> GSHMGTAAEHHREGIMSQFFYIHPDNPQQRLINQAVEIVRKGGVIVYPTDSGYALGCKIEDKNAMERICRIRQLPDGHNFTLMC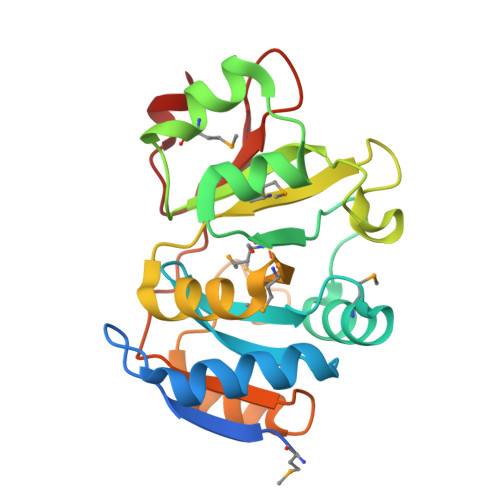RDLSELSTYSFVDNVAFRLMKNNTPGNYTFILKGTKEVPRRLLQEKRKTIGMRVPSNPIAQALLEALGEPMLSTSLMLPGSEFTESDPEEIKDRLEKQVDLIIHGGYLGQKPTTVIDLTDDTPVVVREGVGDVKPFL Human feline leukaemia virus subgroup C receptor-related proteins 1 and 2 (FLVCR1 and FLVCR2) are members of the major facilitator superfamily. Here, we show that FLVCR1 and FLVCR2 facilitate the transport of choline and ethanolamine across the plasma membrane, using a concentration-driven substrate translocation process. Fully conserved tryptophan and tyrosine residues form the binding pocket of both transporters and confer selectivity for choline and ethanolamine through cation–π interactions. Our findings indicate that both FLVCR1 and FLVCR2 operate as uniporters, facilitating downhill ligand transport independent of sodium or pH gradients.

We determined structures of FLVCR1 and FLVCR2 in as-isolated (without exogenous addition of ligands), inward-facing conformations at 2.9 Å resolution. The inward-facing conformations of FLVCR1 and FLVCR2 exhibit a close resemblance to each other, with a root mean square deviation (Cα r.m.s.d.) of 0.993 Å. Both structures feature a wedge-shaped solvent-accessible cavity that is mainly created by the separation of TM4 and TM5 of the N domain from TM10 and TM11 of the C domain. Although FLVCR1 exhibits a similar extracellular hydrogen-bonding network as FLVCR2, it lacks a corresponding salt bridge interaction. Notably, the disruption of the hydrogen bond between N133FLVCR1 and N359FLVCR1 (structurally analogous to N110FLVCR2 and N332FLVCR2) through an alanine substitution of N133FLVCR1 markedly diminishes the transport activity of FLVCR1 for both choline and ethanolamine. Of note, although the as-isolated, inward-facing and outward-facing conformations of FLVCR2 represent apo states of the transporter, we observed an extra non-protein density within the substrate-binding cleft of the as-isolated FLVCR1 structure. Introducing choline and ethanolamine to FLVCR1 leads to displacement of this unidentified molecule, evident from the altered size and shape of the specific densities for choline and ethanolamine in the respective electron microscopy maps. The precise nature of this ligand remains unknown. It is, however, conceivable that FLVCR1 is copurified with a blend of choline and ethanolamine, creating an indistinct density for these ligands or alternatively with a yet-unidentified ligand.

> MARPDDEEGAAVAPGHPLAKGYLPLPRGAPVGKESVELQNGPKAGTFPVNGAPRDSLAAASGVLGGPQTPLAPEEETQARLLPAGAGAETPGAESSPLPLTALSPRRFVVLLIFSLYSLVNAFQWIQYSIISNVFEGFYGVTLLHIDWLSMVYMLAYVPLIFPATWLLDTRGLRLTALLGSGLNCLGAWIKCGSVQQHLFWVTMLGQCLCSVAQVFILGLPSRIASVWFGPKEVSTACATAVLGNQLGTAVGFLLPPVLVPNTQNDTNLLACNISTMFYGTSAVATLLFILTAIAFKEKPRYPPSQAQAALQDSPPEEYSYKKSIRNLFKNIPFVLLLITYGIMTGAFYSVSTLLNQMILTYYEGEEVNAGRIGLTLVVAGMVGSILCGLWLDYTKTYKQTTLIVYILSFIGMVIFTFTLDLRYIIIVFVTGGVLGFFMTGYLPLGFEFAVEITYPESEGTSSGLLNASAQIFGILFTLAQGKLTSDYGPKAGNIFLCVWMFIGIILTALIKSDLRRHNINIGITNVDVKAIPADSPTDQEPKTVMLSKQSESAIDYKDDDDK>[3x]MAHHHHHH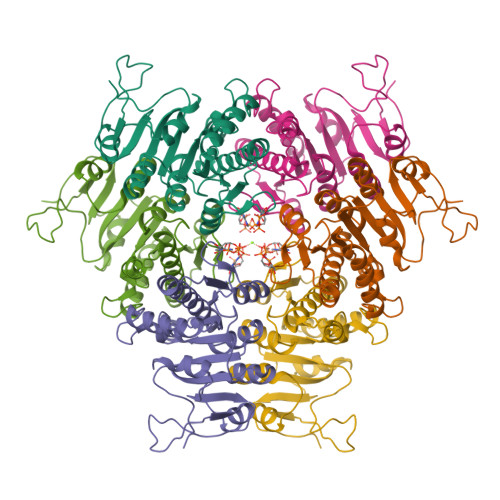MRPYKRVLIKLSGGALADQTGNSFNSKRLEHIANEILSIVDLGIEVSIVIGGGNIFRGHLAEEWGIDRVEADNIGTLGTIINSLMLRGVLTSKTNKEVRVMTSIPFNAVAEPYIRLRAVHHLDNGYIVIFGGGNGQPFVTTDYPSVQRAIEMNSDAILVAKQGVDGVFTSDPKHNKSAKMYRKLNYNDVVRQNIQVMDQAALLLARDYNLPAHVFNFDEPGVMRRICLGEHVGTLINDDASLLVHEK> ETDEEPEEPGRRGSFVEMVDNLRGKSGQGYYVEMTVGSPPQTLNILVDTGSSNFAVGAAPHPFLHRYYQRQLSSTYRDLRKGVYVPYTQGKWEGELGTDLVSIPHGPNVTVRANIAAITESDKFFINGSNWEGILGLAYAEIARPDDSLEPFFDSLVKQTHVPNLFSLQLCGAGFPLNQSEVLASVGGSMIIGGIDHSLYTGSLWYTPIRREWYYEVIIVRVEINGQDLKMDCKEYNYDKSIVDSGTTNLRLPKKVFEAAVKSIKAASSTEKFPDGFWLGEQLVCWQAGTTPWNIFP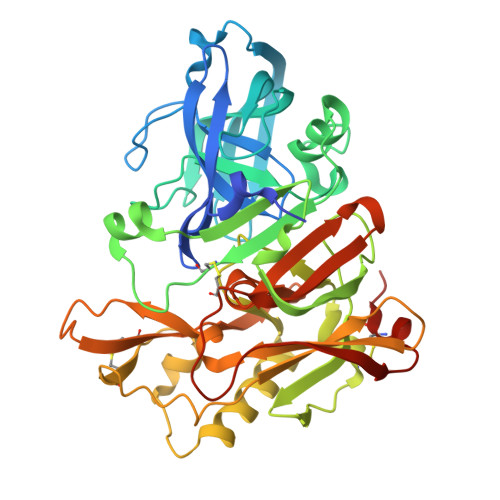VISLYLMGEVTNQSFRITILPQQYLRPVEDVATSQDDCYKFAISQSSTGTVMGAVIMEGFYVVFDRARKRIGFAVSACHVHDEFRTAAVEGPFVTLDMEDCGYNIPQTDEST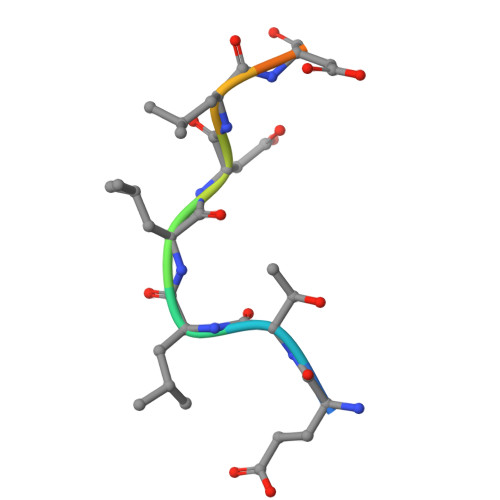> ETLLDLDFDP>[4x]MAKKTSSKGKLPPGPLPLPGLGNLLHVDFQNTPYCFDQLRRRFGDVFSLQLA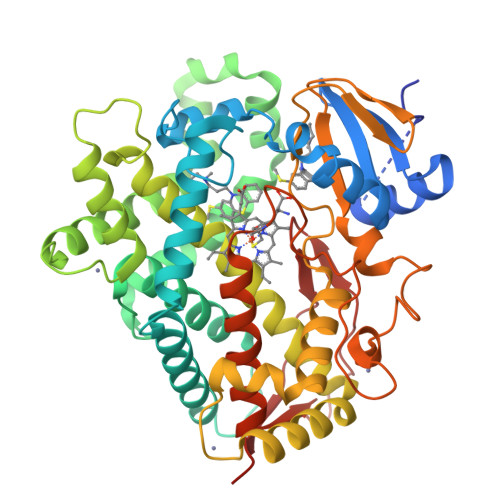WTPVVVLNGLAAVREALVTHGEDTADRPPVPITQILGFGPRSQGVFLARYGPAWREQRRFSVSTLRNLGLGKKSLEQWVTEEAACLCAAFANHSGRPFRPNGLLDKAVSNVIASLTCGRRFEYDDPRFLRLLDLAQEGLKEESGFLREVLNAVPVLLHIPALAGKVLRFQKAFLTQLDELLTEHRMTWDPAQPPRDLTEAFLAEMEKAKGNPESSFNDENLRIVVADLFSAGMETTSTTLAWGLLLMILHPDVQRRVQQEIDDVIGQVRRPEMGDQAHMPYTTAVIHEVQRFGDIVPLGVTHMTSRDIEVQGFRIPKGTTLITNLSSVLKDEAVWEKPFRFHPEHFLDAQGHFVKPEAFLPFSAGRRACLGEPLARMELFLFFTSLLQHFSFSVPTGQPRPSHHGVFAFLVSPSPYELCAVPRHHHH>MGHHHHHHGGTILVVTGTGTGVGKTVVCAALASAAR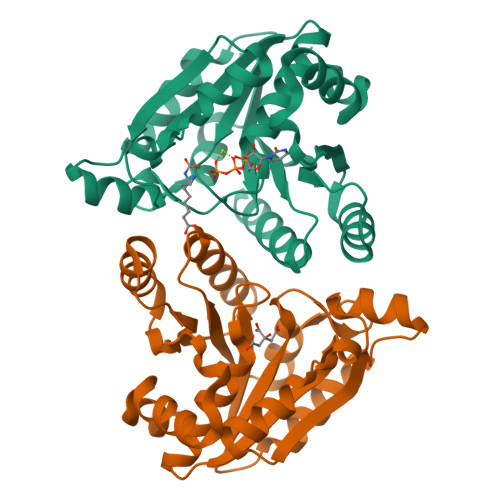QAGIDVAVCKPVQTGTARGDDDLAEVGRLAGVTQLAGLARYPQPMAPAAAAEHAGMALPARDQIVRLIADLDRPGRLTLVEGAGGLLVELAEPGVTLRDVAVDVAAAALVVVTADLGTLNHTKLTLEALAAQQVSCAGLVIGSWPDPPGLVAASNRSALARIAMVRAALPAGAASLDAGDFAAMSAAAFDRNWVAGLVG[4x]> VTTTATLTYPFHDWSQELSPRYAQLRASD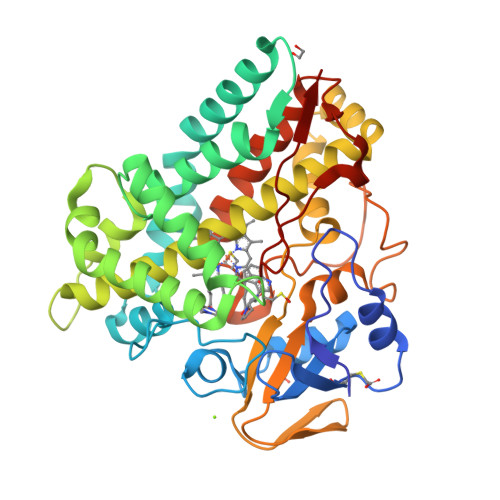APVCPVVSEGTGDPLWLVTRYATAVKLLEDSRFSSEAAIASGAPRQEPVELRAPGTRADGVAMLREAGLRSVLADGLGPRAVRRHQGWINDLAETLMSELASREGTFDLAADFVEPLSSALVSRTLLGELSADERDLLAHCADTGLRFCGVTHEEQVHAFTQMHEFFLEHARRLAGTPGEHLLKLIAEAPVDQGPLSDEALAEAGSLLVVAGFPTSSGFLCGALLTLLRHPDAVQELHAHPERVPSAVEELLRYTPLSTGSVKRMATEDLEIDGVRIKAGEVVMVSLEAVNHDPDAFEDPDVFRPGREGPMHFGFGRGRHFCPGNRLARCVIEATVRAVARRPGLRLAVAPEEISWHEGLFFRRPRAIPATW> MAHAGRTGYDNREIVMKYIHYKLSQRGYEWDAGDVGAAPPGAAPAPGIFSSQPGHTPHPAASRDPVARTSPLQTPAAPGAAAGPALSPVPPVVHLTLRQAGDDFSRRYRRDFAEMSSQLHLTPFTARGRFATVVEELFRDGVNWGR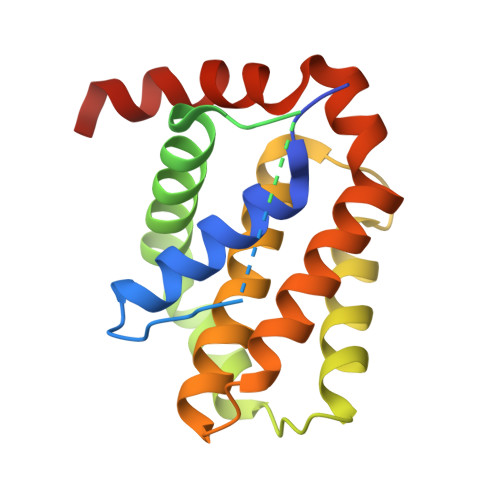IVAFFEFGGVMCVESVNREMSPLVDNIALWMTEYLNRHLHTWIQDNGGWDAFVELYGPSMRLEHHHHHH> MAISLATKAATDALKVNRAPVGVEPQEVHKWLQSFNWDFKENRTKYPTKYHMANETKEQFKVIAKEYARMEAAKDERQFGTLLDGLTRLGAGNKVHPRWGETMKVISNFLEVGEYNAIAASAMLWDSATAAEQKNGYLAQVLDEIRHTHQCAFINHYYSKHYHDPAGHNDARRTRAIGPLWKGMKRVFADGFISGDAVECSVNLQLVGEACFTNPLIVAVTEWASANGDEITPTVFLSVETDELRHMANGYQTVVSIANDPASAKFLNTDLNNAFWTQQKYFTPVLGYLFEYGSKFKVEPWVKTWNRWVYEDWGGIWIGRLGKYGVESPASLRDAKRDAYWAHHDLALAAY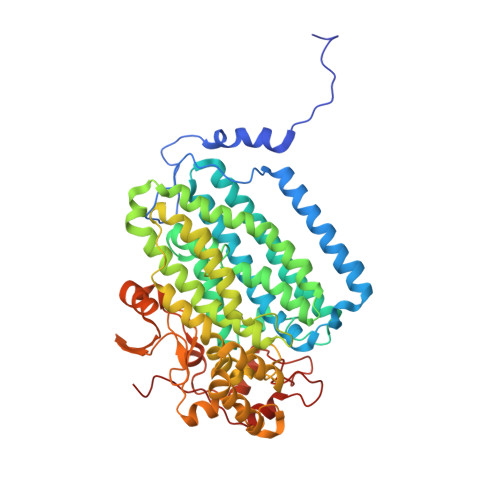AMWPLGFARLALPDEEDQAWFEANYPGWADHYGKIFNEWKKLGYEDPKSGFIPYQWLLANGHDVYIDRVSQVPFIPSLAKGTGSLRVHEFNGKKHSLTDDWGERQWLIEPERYECHNVFEQYEGRELSEVIAEGHGVRSDGKTLIAQPHTRGDNLWTLEDIKRAGCVFPDPLAKF>[6x]GPGSMPSERTFI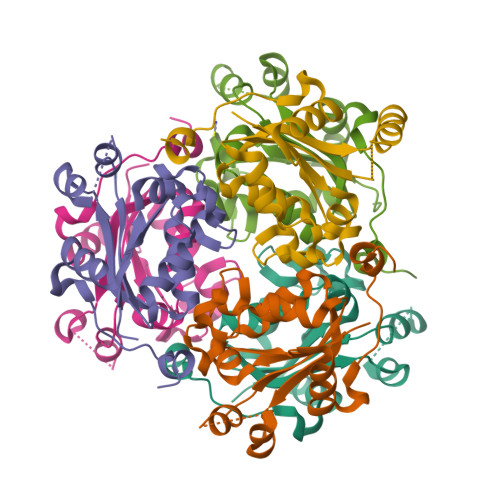AVKPDGVQRNLVGEIIKRFENKGYKLVGLKLLQPTEEQAKQHYIDLASKPFYSGLVSYFSSGPIVGMVWEGLGVVKGGRVLLGATNPADSLPGTIRGDFAVDVGRNVCHGSDSVESAKREIAFWFKAEELVSWTSHSVKQIYERA> TRY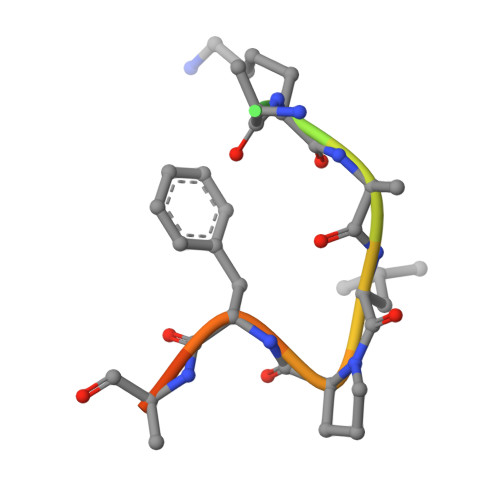WNAKALPFAFGA> GHMGSGSMPEEEKAARLLIEALEKGDPELMRKVISPDTKMSVNGRLFTGDEVVEAVKEIQKRGIVIK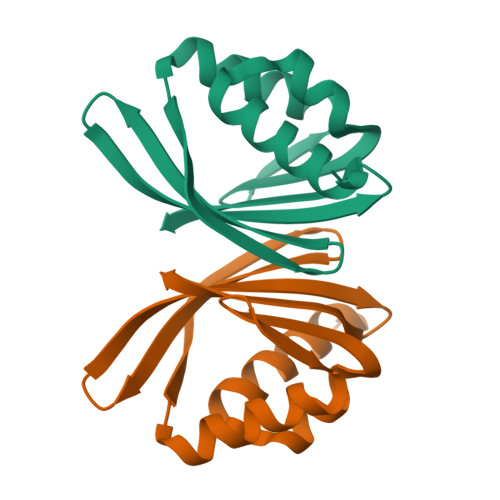LVSYEKAGNLWLFLVTVKNNGQEEKQAVAIVVRNGRIKEVIAMSIK> MSNFINIHVLISHSPSCLNRDDMNMQKDAIFGGKRRVRISSQSLKRAMRKSGYYAQNIGESSLRTIHLAQLRDVLRQKLGERFDQKIIDKTLALLSGKSVDEAEKISADAVTPWVVGEIAWFCEQVAKAEADNLDDKKLLKVLKEDIAAIRVNLQQGVDIALSGRMATSGMMTELGKVDGAM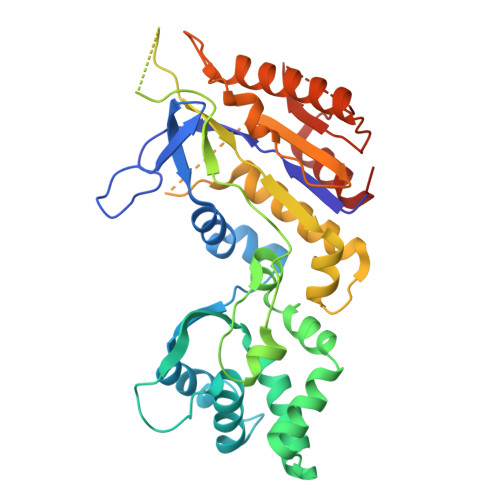SIAHAITTHQVDSDIDWFTAVDDLQEQGSAHLGTQEFSSGVFYRYANINLAQLQENLGGASREQALEIATHVVHMLATEVPGAKQRTYAAFNPADMVMVNFSDMPLSMANAFEKAVKAKDGFLQPSIQAFNQYWDRVANGYGLNGAAAQFSLSDVDPITAQVKQMPTLEQLKSWVRNNGEA> XCELCCNPG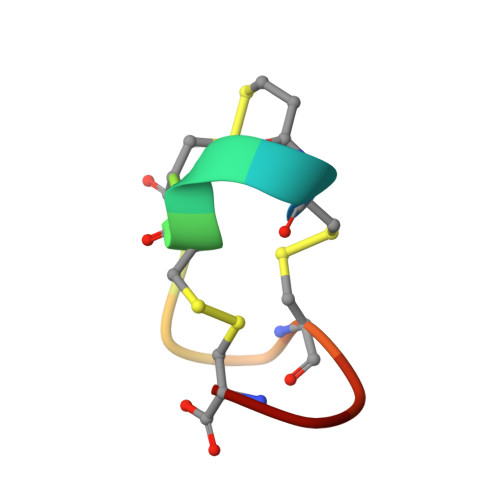CAGC> MSTNLNPFMNNTPSSSPLKGSESKRVSKRPISSSSSASLLSSPSRRSRPSTVYGDRYIPSRTDIDFNSIVSISSMASVPALNPSSTEDQVEYQKERQAHETYNTLLKNELFGEMLSKDTVGSESSIDRIKNTRPSTRGNVHAENTTRHGYELE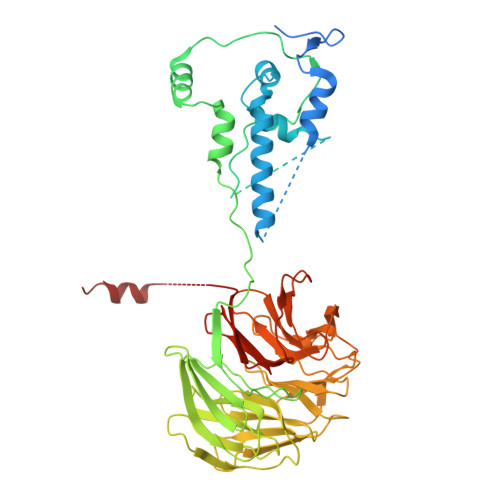RVSTPPPEAAGLEEFSPHSTPVTPRRLFTSQQDEITRPSSNSVRGASLLTYQQRKGRRLSAASLLQSQFFDSMSPVRPDSKQLLLSPGKQFRQIAKVPYRVLDAPSLADDFYYSLIDWSSTDVLAVALGKSIFLTDNNTGDVVHLCDTENEYTSLSWIGAGSHLAVGQANGLVEIYDVMKRKCIRTLSGHIDRVACLSWNNHVLTSGSRDHRILHRDVRMPDPFFETIESHTQEVCGLKWNVADNKLASGGNDNVVHVYEGTSKSPILTFDEHKAAVKAMAWSPHKRGVLATGGGTADRRLKIWNVNTSIKMSDIDSGSQICNMVWSKNTNELVTSHGYSKYNLTLWDCNSMDPIAILKGHSFRVLHLTLSNDGTTVVSGAGDETLRYWKLFDKPKAKVQPNSLIFDAFNQIR>[2x]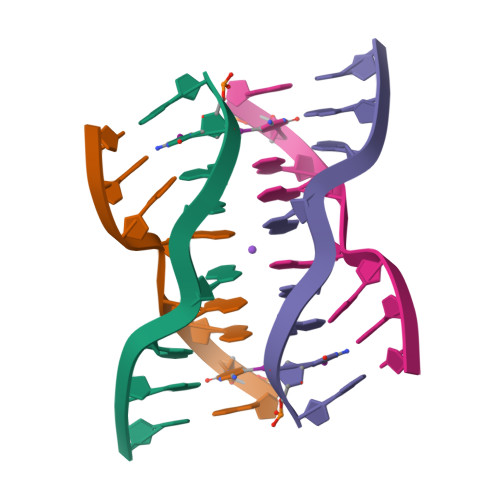GCGAGAGC> TQVCTGTDMKLRLPASPETHLDMLRHLYQGCQVVQGNLELTYVPANASLSFLQDIQEVQGYMLIAHNQVKRVPLQRLRIVRGTQLFEDKYALAVLDNRDPQDNVAASTPGRTPEGLRELQLRSLTEILKGGVLIRGNPQLCYQDM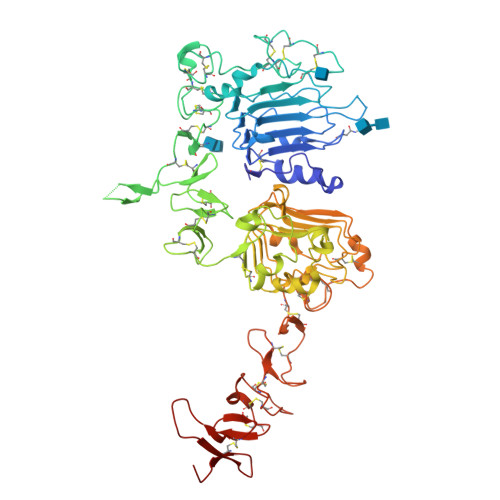VLWKDVFRKNNQLAPVDIDTNRSRACPPCAPACKDNHCWGESPEDCQILTGTICTSGCARCKGRLPTDCCHEQCAAGCTGPKHSDCLACLHFNHSGICELHCPALVTYNTDTFESMHNPEGRYTFGASCVTTCPYNYLSTEVGSCTLVCPPNNQEVTAEDGTQRCEKCSKPCARVCYGLGMEHLRGARAITSDNVQEFDGCKKIFGSLAFLPESFDGDPSSGIAPLRPEQLQVFETLEEITGYLYISAWPDSLRDLSVFQNLRIIRGRILHDGAYSLTLQGLGIHSLGLRSLRELGSGLALIHRNAHLCFVHTVPWDQLFRNPHQALLHSGNRPEEDCGLEGLVCNSLCAHGHCWGPGPTQCVNCSHFLRGQECVEECRVWKGLPREYVSDKRCLPCHPECQPQNSSETCFGSEADQCAACAHYKDSSSCVARCPSGVKPDLSYMPIWKYPDEEGICQPCPIN> GSHMSSLPVPYKLPVSLSVGSCVIIKGTPIHSFINDPQLQVDFYTDMDEDSDIAFRFRVHFGNHVVMNRREFGIWMLEETTDYVPFEDGKQFELCIYVHYNE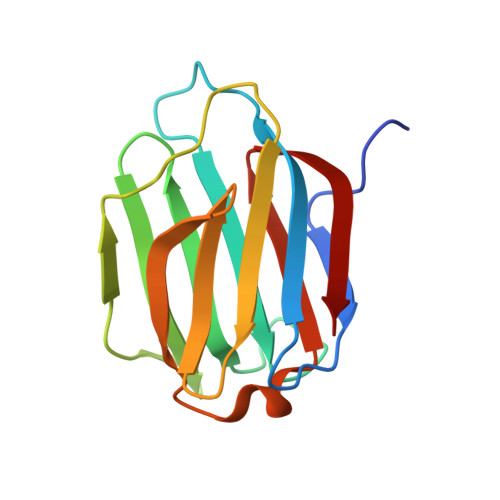YEIKVNGIRIYGFVHRIPPSFVKMVQVSRDISLTSVSVSN> GSSMANNALQTIINARLPGEEGLWQIHLQDGKISAIDAQSGVMPITENSLDAEQGLVIPPFVEPHIHLDTTQTAGQPNWNQSGTLFEGIERWAERKALLTHDDVKQRAWQTLKWQIANGIQHVRTHVDVSDATLTALKAMLEVKQEVAPWIDLQIVAFPQEGILSYPNGEALLEEALRLGADVVGAIPHFE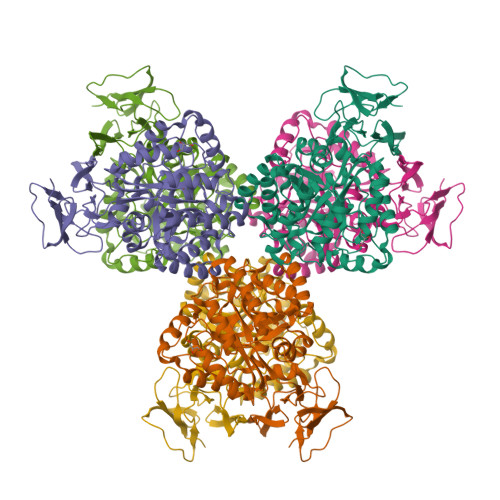FTREYGVESLHKTFALAQKYDRLIDVHCDEIDDEQSRFVETVAALAHHEGMGARVTASHTTAMHSYNGAYTSRLFRLLKMSGINFVANPLVNIHLQGRFDTYPKRRGITRVKEMLESGINVCFGHDSVFDPWYPLGTANMLQVLHMGLHVCQLMGYGQINDGLNLITHHSARTLNLQDYGIAAGNSANLIILPAENGFDALRRQVPVRYSVRGGKVIASTQPAQTTVYLEQPEAIDYKR KtrAB is a cation channel with a nucleotide-dependent RCK domain. The structure of the KtrAB complex revealed a homodimeric membrane protein (KtrB) assembled with a cytosolic RCK octameric ring, formed by the KtrA protein. KtrA binds nucleotides, ATP or ADP. ATP binding induces the adoption of a square-conformation by the octameric ring and increased K+ flux activity through KtrAB; ADP binding results in a non-square conformation and decreased flux.

A simple indicator of ring conformation is the pair of distances (L1 and L2) separating the Cα of N38 residues located in opposite subunits across a ring face. Like in the wild-type protein, the ADP-bound R16K (at 3.0 Å resolution) and R16A (at 3.7 Å resolution) rings adopt a non-square conformation. However, the ADP-bound ring conformations are different from each other and from the wild-type, with L1/L2 distances for the wild-type of 40.7/30.7 Å and for R16K of 52.0/21.9 Å. In the ADP-bound R16A mutant there are eight KtrA dimers present in the asymmetric unit, corresponding to two different rings with L1/L2 distances of 34/30 Å and 37/28 Å.

>MGRIKNKQFAVIGLGAFGGSICKELHRMGHEVLAVDINEEKVNAYASYATHAVIANATEENELLSLGIRNFEYVIVAIGANIQASTLTTLLLKELDIPNIWVKAQNYYHHKVLEKIGADRIIHPEKDMGVKIAQSLSDENVLNYIDLSDEYSIVELLATRKLDSKSIIDLNVRAKYGCTILAIKHHGDICLSPAPEDIIREQDCLVIMGHKKDIKRFENEGM[16x]>MQKAVEITYNGKTLRGMMHLPDDVKGKVPMVIMFHGFTGNKVESHFIFVKMSRALEKVGIGSVRFDFYGSGESDGDFSEMTFSSELEDARQILKFVKEQPTTDPERIGLLGLSMGGAIAGIVAREYKDEIKALVLWAPAFNMPELIMNESVKQYGAIMEQLGFVDIGGHKLSKDFVEDISKLNIFELSKGYDKKVLIVHGTNDEAVEYKVSDRILKEVYGDNATRVTIENADHTFKSLEWEKKAIEESVEFFKKELLKG[6x]

Lipases are enzymes that reversibly catalyze the hydrolysis and synthesis of a large variety of glycerol esters. A minimal lid domain comprising the residues 141-183 is inserted between strand β6 and helix αE on top of the CD active-site area. Different from most other lipases, in which the lid is generally formed by a bundle of α-helices, in Tth MAG lipase this domain is compact. It is formed by two small α-helices, followed by a β-hairpin and an additional α-helix, referred to as α-helix/β-hairpin/α-helix (HBH).

To rule out that the presence of glycerol in the Tth MAG lipase structure is due to the addition of glycerol in the cryo-protectant buffer, we determined an additional Tth MAG lipase structure without using glycerol in any sample preparation step and cryo-protection prior to X-ray data collection. In this structure, glycerol is found in a literally identical active site position in five out of six protein chains of the respective asymmetric unit, confirming its origin to be independent from a specific crystallization and cryo-protection protocol.(2~{S})-2-[[(1~{R},3~{S},4~{S})-2-[(2~{R})-2-[2-(oxidanylamino)-2-oxidanylidene-ethyl]heptanoyl]-2-azabicyclo[2.2.1]heptan-3-yl]carbonylamino]-2-phenyl-ethanoic acid | C24 H33 N3 O6 | 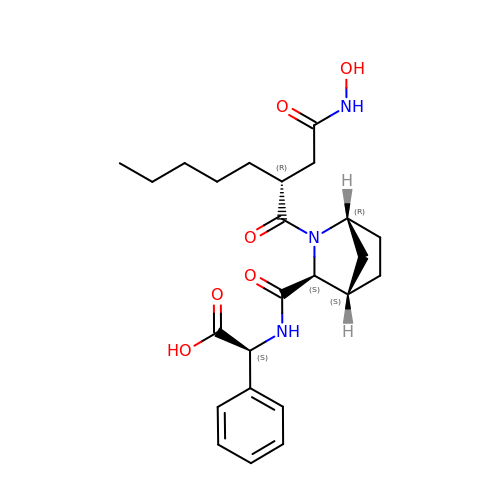ZLHWZWQYBXYOER-SOMHSPELSA-N The de novo pathway of cysteine biosynthesis requires the conversion of O-acetyl-l-serine into l-cysteine, which is catalysed by cysteine synthase (CS). As CS is not found in humans, it constitutes a potential drug target. Crystal structures of the three enzymes were determined at resolutions of 1.80 Å for TcCS, 1.75 Å for LiCS and 2.75 Å for TthCS. These three homodimeric structures show the same overall fold and demonstrate that the active-site geometry is conserved, supporting a common reaction mechanism.

The crystal structure of the TthCS dimer also reveals an extensive dimer interface with buried surface areas of 3053 Å2 for chain A and 3099 Å2 for chain B. The observation that 25% of the protein is involved in dimer interactions clearly indicates that the enzyme is a functional homodimer. In each chain of TthCS continuous electron density was found which fits the structure of the cofactor. Therefore, in this structure the covalently bound state of PLP has been captured. The PLP is located between α1 and α5. The holo form of TthCS confirms the residues involved in binding PLP. TcCS and TthCS both have PLP bound in the active site and therefore represent holo forms of the enzyme. PLP and OAS were not added to either protein during expression or purification and were likely to have been scavenged from the E. coli cells in which the protein was expressed. In contrast, LiCS forms an apo CS structure as no PLP is bound in the active site. The LiCS structure and chain A of TcCS are in the open form, whereas chains B, C and D of TcCS and TthCS are in the closed form.

>[2x]MGSSHHHHHHSSGLVPRGSMSGQEFNKQNDVAPSVDALIGNTPAVYLRNMNKTAATIVLKLESENPMASVKDRLAYAIYDKAEKEGKIKRGKSVIVEATSGNTGIALALLGAVRGYKVIITMPDSMSMERRSLLRIFGAELILTPASLGMKGAVAMANRIVSNNPDAVLADQFCTKYNAQIHEETTGPEIWRQTKGHVDCFVAGVGTGGTLTGVARFLKSVGCNANIVAVEPQESPVLSGGRPGPHRIQGIGAGFVPEVLDRELVDEIIQVSSDKAIETAQKLSRMDGIFCGFSAGANVFAALKIAERPEMAGKTIVTVIPSFGERYLSTALYASVREEITSLPVVPVSEIPQV>[2x]NVQFSNQDGALGEPANYTQFQHVLTESELQISDAEGKKGNKEYFALDGNFTGIVNQYFYVDKKSEALVFKMKNDHLRNEVRVHKNFRTDLPNKLYTLSAEVEIIDPVASMKNSNSKQNEITFLQVANKGLDNQGTHNVPHPLLRVVWKEDANSVKGHFWAMVKNNAVICKGSFGKKNKDKEMCKADVAYKKYDLGKAPLNKATAFDITVGNKQLIIDVDGKRLVEHDIDYWR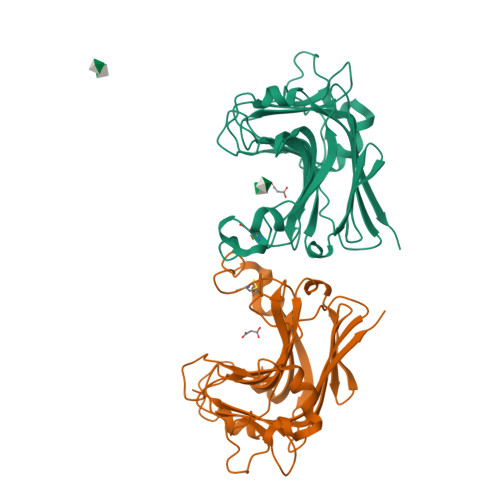HLLSYFKAGVANQFTNGMSEAHFNKLEYKALETK> GHMAVGSTSVYGDALGEVYDLFYRGRGKDFAAEAEWVRRVVRERRPGARSLLDVACGTGEHLAHLVEHFPDAAGVELSPAMRAAAERKLTATPVHQADMFDFDLGRVFDAVCCLTGSIAYAADTAELARAVRAMARHLPVGGVLVIDPWWSPGTFLDGHIAH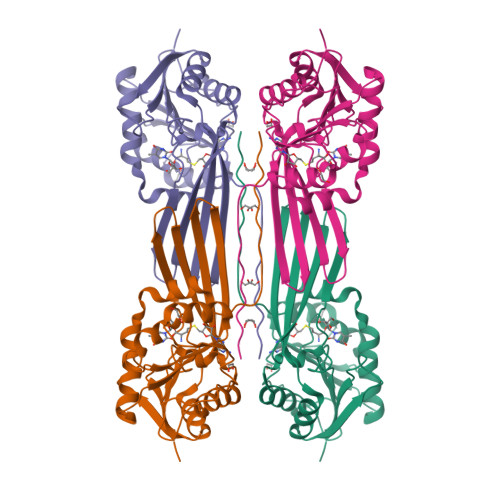DVVEGEGRTVVRLSRSHRIGDVSRHEAHYLAADATGVRHFSQVQDLTLFPAEDYLAALAAAGCEPEHLTDVGQPRRGLFVGVRREGGR4-{[(1R,2S,3R,5Z,7E,14beta,17alpha)-1,3,25-trihydroxy-9,10-secocholesta-5,7,10-trien-2-yl]oxy}butanenitrile 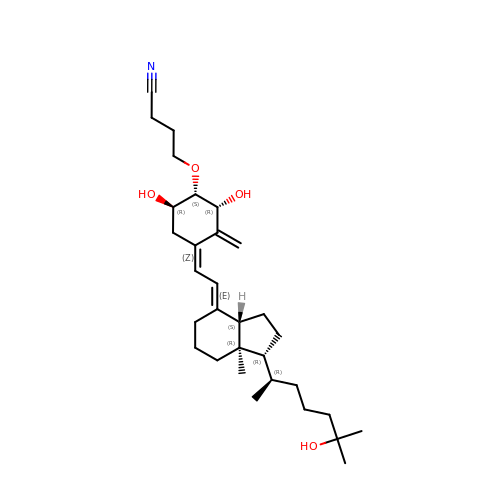| C31 H49 N O4 | KQWXEWOYVIUCOD-IBOBMRDDSA-N>[2x]GDERFYAEHLMPTLQGLLDPESAHRLAVRFTSLGLLPRARFQDSDMLEVRVLGHKFRNPVGIAAGFDKHGEAVDGLYKMGFGFVEIGSVTPKPQEGNPRPRVFRLPEDQAVINRYGFNSHGLSVVEHRLRARQQKQAKLTEDGLPLGVNLGKNKTSVDAA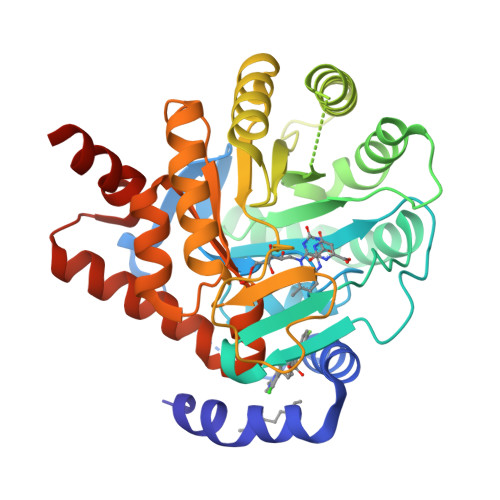EDYAEGVRVLGPLADYLVVNVSSPNTAGLRSLQGKAELRRLLTKVLQERDGLRRVHRPAVLVKIAPDLTSQDKEDIASVVKELGIDGLIVTNTTVSRPAGLQGALRSETGGLSGKPLRDLSTQTIREMYALTQGRVPIIGVGGVSSGQDALEKIRAGASLVQLYTALTFWGPPVVGKVKRELEALLKEQGFGGVTDAIGADHRRLEAGHHHHHH>TVPDNLKKQLAVSVRNIQWSYGIFWSVSASQPGVLEWGDGYYNGDIKTRKTIQAAEVKIDQLGLERSEQLRELYESLSLAESSASGSSQVTRRASAAALSPEDLTDTEWYYLVCMSFVFNIGEGIPGGALSNGEPIWLCNAETADSKVFTRSLLAKSASLQTVVCFPFLGGVLEIGTTEHIKEDMNVIQSVKTLFLEA[6x];>PNVKRGNFTEQEEDLIIRLHKLLGNRWSLIAKRVPGRTDNQVK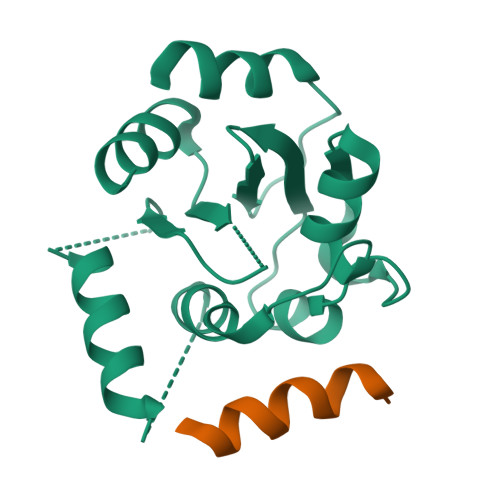NYWNTHLSKKL[6x]> GPLGSMGERFFRNEMPEFVPEDLSGEEETVTECKDSLTKLLSLPYKSFSEKLHRYALSIKDKVVWETWERSGKRVRDYNLYTGVLGTAYLLFKSYQVTRNEDDLKLCLENVEACDVASRDSERVTFICGYAGVCALGAVAAKCLGDDQLYDRYLARFRGIRLPSDLPYELLYGRAGYLWACLFLNKHIGQESISSERMRSVVEEIFRAGRQLGNKGTCPLMYEWHGKRYWGAAHGLAGIMNVLMHTELEPDEIKDVKGTLSYMIQNRFPSGNYLSSEGSKSDRLVHWCHGAPGVALTLVKAAQVYNTKEFVEAAMEAGEVVWSRGLLKRVGICHGISGN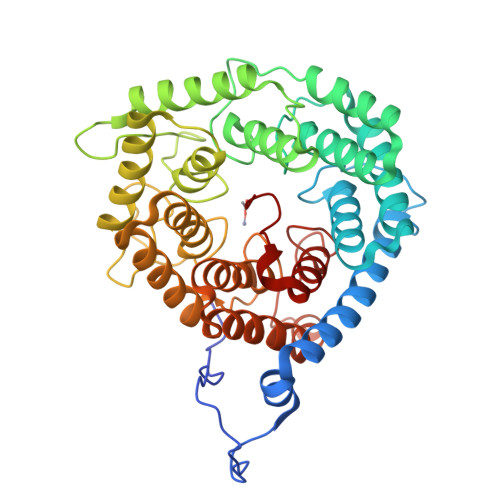TYVFLSLYRLTRNPKYLYRAKAFASFLLDKSEKLISEGQMHGGDRPFSLFEGIGGMAYMLLDMNDPTQALFPGYEL>MGEPRSQPPVERPPTAETFLPLSRV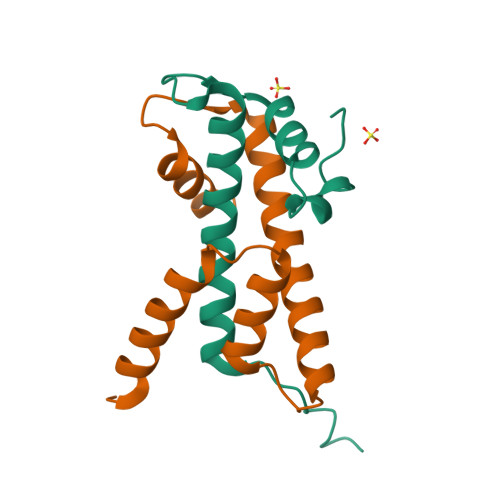RTIMKSSMDTGLITNEVLFLMTKCTELFVRHLAGAAYTEEFGQRPGEALKYEHLSQVVNKNKNLEFLLQIVPQKIRVHQFQEMLRLNRSAGSDDDDDDDDDDDEEESESESESDE[2x];>[2x]MVERIEDLNLPNAVIGRLIKEALPESASVSKEARAAIARAASVFAIFVTSSSTALAHKQNHKTITAKDILQTLTELDFESFVPSLTQDLEVYRKVVKEKKESKASKKDSNTAENANASATATAEEAPE>MGNNLMQTDLSVWGMYQHADIVVKCVMIGLILASVVTWAIFFSKSVEFFNQKRRLKREQQLLAEARSLNQANDIAADFGSKSLSLHLLNEAQNELELSEGSDDNEGIKERTSFRLERRVAAVGRQMGRGNGYLATIGAISPFVGLFGTVWGIMNSFIGIAQTQTTNLAVVAPGIAEALLATAIGLVAAIPAVVIYNVFARQIGGFKAMLGDVAAQVLLLQSRDLDLEASA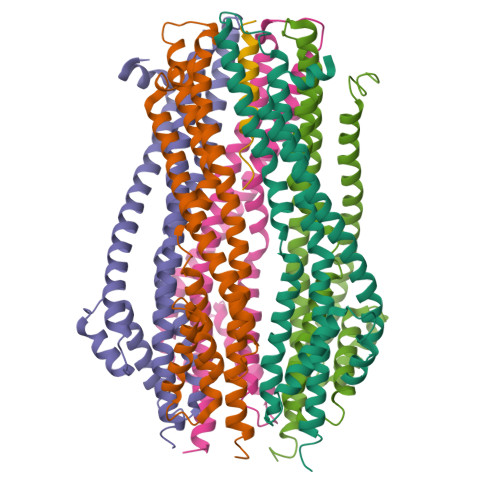AAHPVRVAQKLRAG[5x];> NVTPFIDVMLVLLIIFMVAAPL>GSHMDSAQSDLKEVMVLNATESFVYEPKEQKKMFHATVATENEVFRVKVFNIDLKEKFTPKKIIAIANYVCRNGFLEVYPFTLVADVNADRNMEIPKGLIRSASVTPKINQLCSQTKGSFVNGVFEVHKKNVRGEFTYYEIQDNTGKMEVVVHGRLTTINC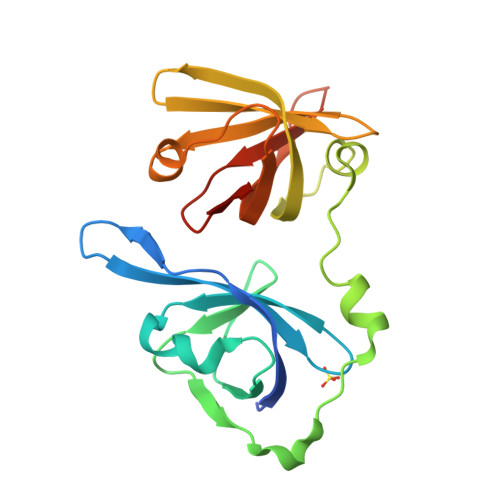EEGDKLKLTCFELAPKSGNTGELRSVIHSHIKVIKTRKN[2x]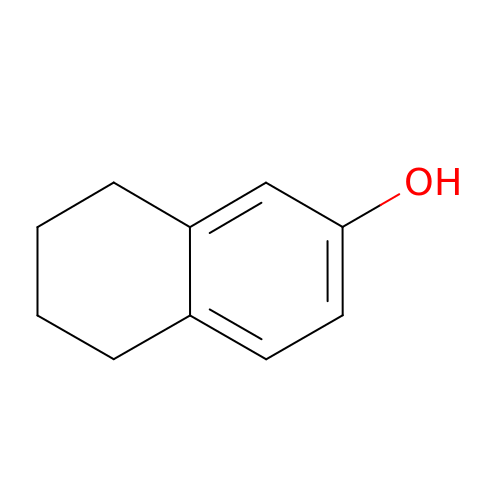5,6,7,8-tetrahydronaphthalen-2-ol | C10 H12 O | UMKXSOXZAXIOPJ-UHFFFAOYSA-N>FTLIELMIVIAIVGILAAVALPAYQDYTARAQVSEAILLAEGQKSAVTEYYLNHGKWPENNTSAGVASSPTDIKGKYVKEVEVKNGVVTATMLSSGVNNEIKGKKLSLWARRENGSVKWFCGQPVTRTDDDTVADAKDGKEIDTKHLPSTCRDNFDAK[5x];>MAAPAVKSASTPKKATAQFLWEAKTKSGESKKGEMEAMDVEAVNARLKSLGLNPVKVRKKSMLDGDITIPGFGGVEGKDILVFTRQFATMIDAGLPLVQCLDILASQMDNPSFKKVLFAIKSKVEQGSTFADALKEHPKVFDELYVQLCAAGEVGGILDAILNRLAAYREKNEKLKSKVKSAMTYPIIVILVAIGVTAVLLLKVTPVFEKMFADFGSELPGPTQMIVNFSHMAQEYFFHVAGSIVAVVMSFTWSYRQPRGRKFWDKVFLFMPVFGPVLRKVAVARFTRTLGTMISSGVPILDALDVTAKTAGNRTVEDAIIYVRGKIAEGKNIAGPLAETKVFPSMVVQMIGVGEATGAMDTMLNKIADFYDDEVDAAINSLTAMIEPVLMVFLGGVVGGFLIGMYLPIFSLAGAIQ[2x];>[12x]MVRGSRPSGGQAGSRHFLGGVDGQCYAGCLSTESRMAKGKLVLGLDIGSTSIKMILLKEQRKRGEVIYALQSFGMKPLPPEAIVDGALMNSTAIVQAVQDLMSELKVKGKDVAIGVSGHSVIIKKIQMPRMSQDELEESIQWEAEQYIPFDVKDVNIDTQILDGGGNDATGQMDVLLVAAKKDMINDYTTVVSEAGLAPVVVDVDAFAVQNMFSVNYDVPERETVVLINAGASVVNINIISNGATVFTRDVTIGGNQFTEEIQKQLNVSYEEAEALKIGGNGADADAVVPQDVERVLSSVAEQVAGEIQRSLDFYAGTAADSNFSKVYLSGGTAKIPALFKTIEARTGVPVEILNPFRKIEVDNRKFDPAFVMDVAPMAAVAVGLALRRPGDKLA;>MMIRINLLPVRAVKKREMGRQVLVLFAVVLIGAGVANYLWYDDRQSELEAHQAGVASTKARIAELEKIIGEVKNINTRKAEVEKKLAVLDALRKGRSGPVRMMDALASATPKKVWVKTFSENNNAVSIDGSAVSHDEVAEFMRGLNGVVWTPKGMGRLVDRRRDSKTARVEMLTSDATIEEFPEAQVSPFFKNIDLQTAKQVGGAQVGVPILVEFKITMTSNYAI[12x];>MDKYLDQFVKAPPAIKFGGLAFVVGALTAANFFMVIQPTEEEIGWAVAERRKLDLELADKSEIAQNLNERRREMDVLEQKLSEALTELPEQRDIEELLAQINDIGKKSGLELSSVTPGKESVGGGEFFARIPIKMTVSGNYHEIALFLQEMANMRRIVNVNNIKFDSAKLKNEKVVLQSEFQATTFRFVEQKAAASTAGNSNSKK[12x];>MLAACEEPPAPAPPPAKPKAAAAVPVKAAPTETGAQAAPSYSYVYNPVGKRDPFRSPIDELGPVNANPVAACNEPLCSFDLDQLKLVAVVTGDASPVAMVEDPAGRGHIVRRNTRMGRQGGKVTQILRDSVTVTEVFSGNGEIIKNPVTLQLKPDAKQDPAYNMMTGRNYGE[12x];>MLEESAVTRGKWMLAAAWAVVLVGARVHGAELNTLRGLDVSRTGSGAQVVVTGTRPPTFTVFRLSGPERLVVDLSSADATGIKGHHEGSGPVSGVVASQFSDQRASVGRVLLALDKASQYDVRADGNRVVISVDGTSQSVDAKRAETPARTERMTASVEAKPHPVAAQAPAKVVKAESAAVPKAALPENVVAAEADEREVSNPAQHITAMSFADDTLSIRADGDIARYEVLELADPPRLAVDLFGVGLATRAPRVKSGALRDVRVGAHADKVRLVLDVRGTMPAYRVDRANRGLEVVLGRAVARTWRRPLRPRAVVASVAEVEPLRQTPVKSDASPVVEVKDVRFEESSSGGRIVMKLSGTSGWKVDRPDPRSAVLTLDNARLPKKFERSLDTSALDTPVKMISAFSVPGAGGKVRLVVAADGAIEEKVSQSAGTLSWRLDVKGVKTEEVAVAQRTAGFTTEAPAYAAEGAPQQARYRGKRVSFEFKDIDIQNLLRVIAEISKKNIVVADDVSGKVTIRLRNVPWDQALDLVLRTKALGKEEFGNIIRIAPLKT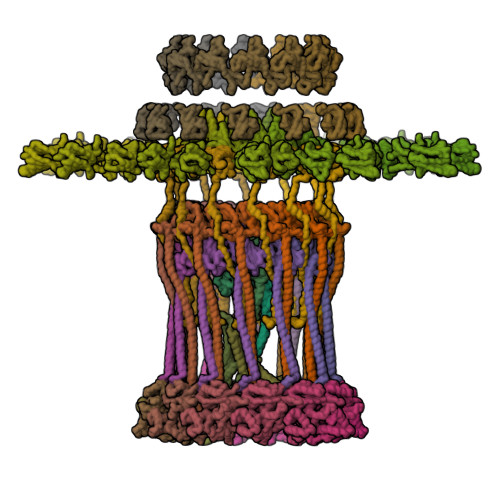LEEEARLRQERKKSLQQQEDLMVNLLPVNYAVAADMAARVKDVLSERGSVTVDQRTNVLIVKDVRSNTERARSLVRSLDTQTPQVLIESRIVEANTSFSRSLGVQWGGQARAGQATGNSTGLIFPNNLAVTGGVTGTGAGLPDNPNFAVNLPTGTGQGVGGAMGFTFGSAGGALQLNLRLSAAENEGSVKTISAPKVTTLDNNTARINQGVSIPFSQTSAQGVNTTFVEARLSLEVTPHITQDGSVLMSINASNNQPDPSSTGANGQPSIQRKEANTQVLVKDGDTTVIGGIYVRRGATQVNSVPFLSRIPVLGLLFKNNSETDTRQELLIFITPRILNRQTIAQTL[12x];>[12x]MMLLSKGRPAMRSRILTSLMLSLAVAPTAYAQQENEEEQDTGGEMGGAEVMDEAPDSAPPTSVAMPPGAPRGRESAPGEVHSVESGDTLWDLSQRYLGSPWYWPKVWSYNPEIANPHWIYPGNQVRFFAAGEEVPTQVTEMVVDEGDVTAPMEMTSNDQVIVTGKIGVDLANSVPVTTQGFVTQRELDEAGRIEGSPSNAVMLSFPDSVYVRFKRKGDVKVGDRYVVYHTTQAVKHPVTGRPLGFLTDFVGTLRVQRVGDGIVTAQIMDTWDGIERGDLVGPVGERLTERVAPKPNAKQVDGTVITALVPYLTVLGENHSIVVDKGSADGVELGNTFNILRKGDPSRHVLGHDVRKPSKEEQSFPWRSIGACMVTEVKERTSNCLMTRSLEELVPGDRAHMSAGASPSASR>MSFPYFISPEQAMRERSELARKGIARAKSVVALAYAGGVLFVAENPSRSLQKISELYDRVGFAAAGKFNEFDNLRRGGIQFADTRGYAYDRRDVTGRQLANVYAQTLGTIFTEQAKPYEVELCVAEVAHYGETKRPELYRITYDGSIADEPHFVVMGGTTEPIANALKESYAENASLTDALRIAVAALRAGSADTSGGDQPTLGVASLEVAVLDANRPRRAFRRITGSALQALLVDQESPQSDGESSG[14x];>MVIGLSTGSDDDDVEVIGGVDPRLIAVQENDSDESSLTDLVEQPAKVMRIGTMIKQLLEEVRAAPLDEASRNRLRDIHATSIRELEDGLAPELREELDRLTLPFNEDAVPSDAELRIAQAQLVGWLEGLFHGIQTALFAQQMAARAQLQQMRQGALPPGVGKSGQHGHGTGQYL[14x];>[14x]TTIVALKYPGGVVMAGDRRSTQGNMISGRDVRKVYITDDYTATGIAGTAAVAVEFARLYAVELEHYEKLEGVPLTFAGKINRLAIMVRGNLAAAMQGLLALPLLAGYDIHASDPQSAGRIVSFDAAGGWNIEEEGYQAVGSGSLFAKSSMKKLYSQVTDGDSGLRVAVEALYDAADDDSATG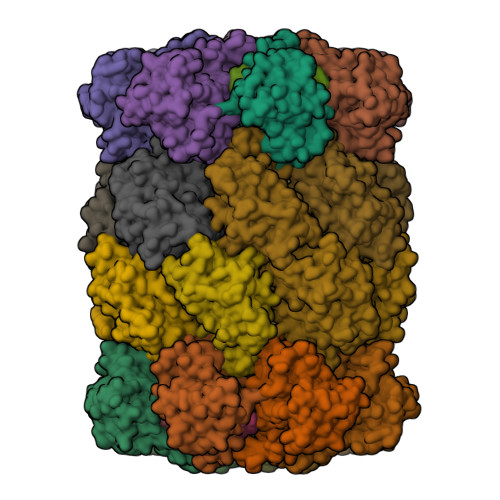GPDLVRGIFPTAVIIDADGAVDVPESRIAELARAIIESRSGADTFGSDGGEKHHHHHH>AIDEIKSRGYLLVGLSADFPPFEFVDENGNIVGFDVDLAKEIARRLGVELKIVDMTFDGLIPSLLTKKIDVIISGMTITEERKKVVAFSDPYFDAGQVIVVRKDSDFRPKTYEDLVGKTVAVQIGTTGDIEVSKYDGIKVVRFDKFTDAFLELKRGRADAVVLDSATARAFVAKNPDLVISSG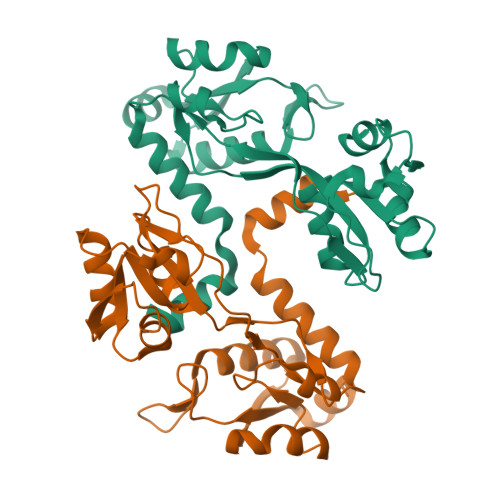VLSSEQYGIAVRKEDTDLLEFINSVLRELKKSPYDVLIEKWFSE[2x]> MAKQNLKSTDRAVQQMLDKAKREGIQTVWDRYEAMKPQCGFGETGLCCRHCLQGPCRINPFGDEPKVGICGATAEVIVARGLDRSIAAGAAGHSGHAKHLAHTLKKAVQGKAASYMIKDRTKLHSIAKRLGIPTEGQKDEDIALEVAKAALADFHEKDTPVLWVTTVLPPSRVKVLSAHGLIPAGIDHEIAEIMHRTSMGCDADAQNLLLGGLRCSLADLAGCYMGTDLADILFGTPAPVVTESNLGVLKADAVNVAVHGHNPVLSDIIVSVSKEMENEARAAGATGINVVGICCTGNEVLMRHGIPACTHSVSQEMAMITGALDAMILDYQCIQPSVATIAECTGTTVITTMEMSKITGATHVNFAEEAAVENAKQILRLAIDTFKRRKGKPVEIPN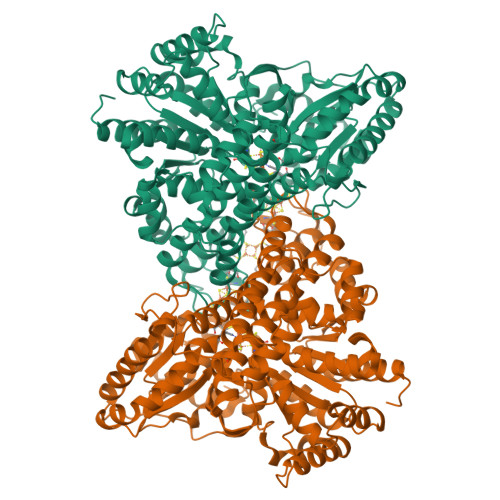IKTKVVAGFSTEAIINALSKLNANDPLKPLIDNVVNGNIRGVCLFAGCNNVKVPQDQNFTTIARKLLKQNVLVVATGCGAGALMRHGFMDPANVDELCGDGLKAVLTAIGEANGLGGPLPPVLHMGSCVDNSRAVALVAALANRLGVDLDRLPVVASAAEAMHEKAVAIGTWAVTIGLPTHIGVLPPITGSLPVTQILTSSVKDITGGYFIVELDPETAADKLLAAINERRAGLGLPW> MDKYTALIHDENFSTLTLNVSRYPKSLAYWEKLLNYIVKASAPICKSTEPQLLKLIRCTYSSMLNEFPYLENYYIDFALLEYKLGNVSMSHKIFQRGLQAFNQRSLLLWTSYLKFCNNVISHQKQLFKKYETAEEYVGLHFFSGEFWDLYLEQISSRCTSSKKYWNVLRKILEIPLHSFSKFYALWLQRIDDIMDLKQLSQLTSKDELLKKLKIDINYSGRKGPYLQDAKKKLKKITKEMYMVVQYQVLEIYSIFESK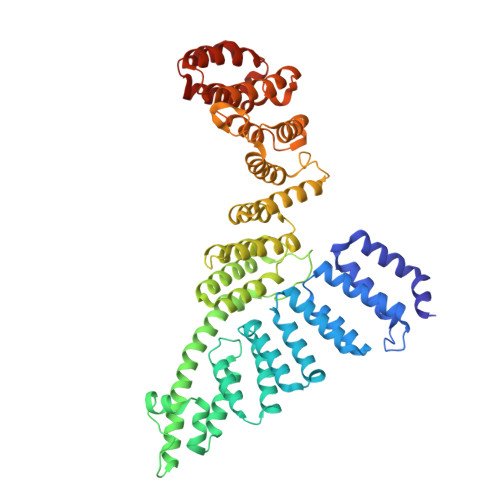IYINYYTSPETLVSSDEIETWIKYLDYTITLQTDSLTHLNFQRALLPLAHYDLVWIKYSKWLINSKNDLLGAKNVLLMGLKFSLKKTEIIKLLYSVICKLNEYVLLRNLLEKIESSYSDNVENVDDFEIFWDYLQFKTFCQNSLYSSRYSDSQSNGLLNKELFDKVWKRLSCKEKKSGQEILLNNLVQFYSKDTVEFVEKNIFQKIIEFGWEYYLQNGMFWNCYCRLIYFDTSRSYLDKRQYIVRKIWPQIDKKFAQSVLPSLTEFCESYFPEEMDTLEEMFTEEP> MEK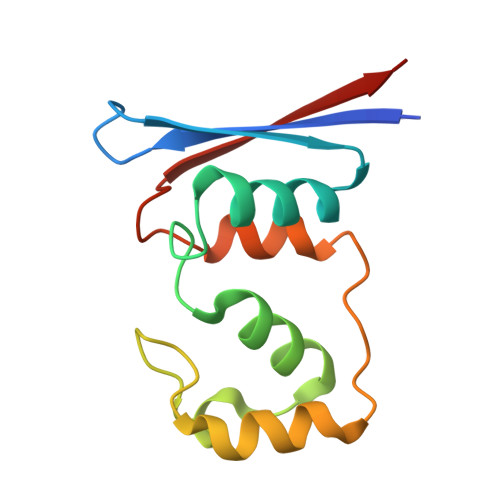VDTWIVYRGRTADMNKSYIAEGSTYEEVYNNFVDKYGYDVLDEDIYEIQLLKKNGENLDDYDVDSDGINNYDKLDEFRESDYVDLEDYDYRELFENSSSQVYYHEFEITHE Pks13 is a multidomain enzyme that performs the final step in the synthesis of mycolic acids through the condensation of a long-chain fatty acid (C24–C26) and a very long-chain fatty acid (C56).12 The product is transferred from Pks13 to trehalose by the Pks13-TE domain. Pks13 fulfills a critical function for Mtb by performing a condensation reaction of a long-chain fatty acid and a very long-chain meromycolic acid to form a mycolic acid. Pks13-TE is a validated target for the development of antibiotics for Mtb. In previous work, we identified TAM16, a potent lead molecule for Pks13-TE. X-ray crystallography verified that compounds from all three different series were binding deep within the active site of Pks13-TE, displacing the side chain of Arg1563 with atoms within about 4 Å from the catalytic Ser1533 OG.

Pks13-TE was preincubated with X20404 (series 1) prior to crystallization. Crystals were in the same P21212 space group as previously reported for the TAM16 complex. There were two molecules of protein per asymmetric unit, each bound to one inhibitor. The crystals diffracted to a resolution of 2.1 Å. Unlike TAM16, which inhibits by blocking the entrance to the catalytic center of Pks13-TE, X20404 binds closely to the catalytic serine (C23 of the X20404 is 3.25 Å from Ser1533 OG) and engages more extensively with the enzyme in a hydrophobic channel that likely binds the alkyl chain of the mycolic acid. This channel passes through the central core of the enzyme, extending from one solvent-accessible side of Pks13-TE to the other. The channel occupied by X20404 was not completely visible in the Pks13-TE-TAM16 structure because the side chain of Arg1563 blocked it. To accommodate the R2 group of X20404 required the displacement of the Arg1563 side chain, and an entire segment of the protein from Thr1645 to Gln1649 is also shifted by approximately 2.4 Å (as measured at CA of Thr1645) to open the channel compared to the TAM16 bound structure, as shown in Figure 3C. Four hydrogen bonds contribute to the binding energy through the following interactions: O29 of R1 with NE2 of His1664; N16 of pyridine of R1 interacts with water connected to the backbone NH of Ala1564 and, through one more water, to the NE of the Arg1563 side chain. The Phe1670s side chain, which flips to stack with the benzofuran core of TAM16, is positioned to form edge-on pi stacking interactions with the R2 phenyl of X20404.

>SNAQIDGFVRTLRARPEAGGKVPVFVFHPAGGSTVVYEPLLGRLPADTPMYGFERVEGSIEERAQQYVPKLIEMQGDGPYVLVGWSLGGVLAYACAIGLRRLGKDVRFVGLIDAVRAGEEIPQTKEEIRKRWDRYAAFAEKTFNVTIPAIPYEQLEELDDEGQVRFVLDAVSQSGVQIPAGIIEHQRTSYLDNRAIDTAQIQPYDGHVTLYMADRYHDDAIMFEPRYAVRQPDGGWGEYVSDLEVVPIGGEHIQAIDEPIIAKVGEHMSRALGQIEADRTSEVGKQ[2x]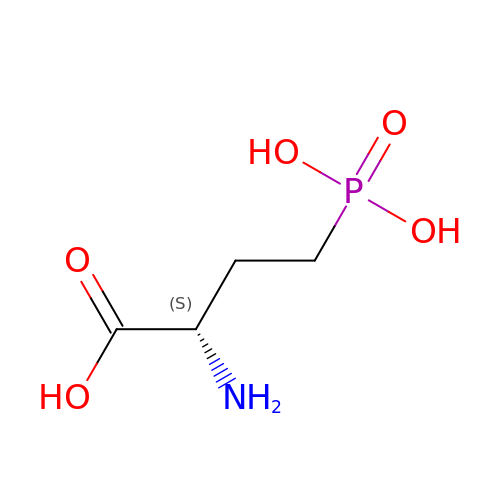(2S)-2-amino-4-phosphonobutanoic acid | C4 H10 N O5 P | DDOQBQRIEWHWBT-VKHMYHEASA-N TAPL is a lysosomal ATP-binding cassette transporter that translocates a broad spectrum of polypeptides from the cytoplasm into the lysosomal lumen. TAPL is a homodimeric half-transporter composed of a transmembrane domain (TMD) and a cytoplasmic nucleotide-binding domain (NBD) with an N-terminal TMD (TMD0). Here we report that, in addition to its well-known role as a peptide translocator, TAPL exhibits an ATP-dependent phosphatidylserine floppase activity that is the possible cause of its high basal ATPase activity and of the lack of coupling between ATP hydrolysis and peptide efflux. Here, we present the cryo-EM structures of mouse TAPL lacking the N-terminal TMD0 in (i) phospholipid-bound, (ii) both CHS- and 9-mer peptide-bound, and (iii) ADP·BeF3-bound states at 3.2–4.0 Å resolutions.

To obtain a nucleotide-bound structure, nanodisc-reconstituted ΔTMD0 was mixed with 9-mer peptide and Mg2+/ADP·BeF3 (mimicking the pre-hydrolysis state) before preparing cryo-EM grids. The final map has a resolution of 3.2 Å, allowing accurate modeling of the Mg2+/ADP·BeF3 complex and side chain conformations. The structure represents the typical outward-facing shape of ABC transporters, in which the two NBDs come close together and the TM helices have a very wide opening towards the lysosomal lumen (~36 Å in the longest diameter), while they are tightly packed on the cytosolic side. As a consequence, ΔTMD0 forms a V-shaped substrate transport pathway open not only to the lysosomal lumen but also laterally to the membrane luminal leaflet. We did not observe any density corresponding to lipids or peptides, indicating that both substrates are exported from ΔTMD0 prior to ATP hydrolysis. In the dimer interface, T286, S287, T290, D294, and Q298 on TM 7 interact electrostatically to stabilize the outward-facing conformation. Interestingly, the F449 residues remain protruding towards the transport pathway and pack closely together to create a latch-like architecture. Consequently, the central cavity is completely isolated from solvent, thus probably preventing the expelled substrate from re-entering. In the NBD region, the two ADP·BeF3 molecules are sandwiched between the two NBDs. The α- and β-phosphates of ADP and BeF3 interact with the Walker A motif and Q-loop from one NBD and the ABC signature motif of the other NBD.

>[2x]MRLWKAVVVTLAFVSTDVGVTTAIYAFSHLDRSLLEDIRHFNIFDSVLDLWAACLYRSCLLLGATIGVAKNSALGPRRLRASWLVITLVCLFVGIYAMAKLLLFSEVRRPIRDPWFWALFVWTYISLAASFLLWGLLATVRPDAEALEPGNEGFHGEGGAPAEQASGATLQKLLSYTKPDVAFLVAASFFLIVAALGETFLPYYTGRAIDSIVIQKSMDQFTTAVVVVCLLAIGSSLAAGIRGGIFTLVFARLNIRLRNCLFRSLVSQETSFFDENRTGDLISRLTSDTTMVSDLVSQNINIFLRNTVKVTGVVVFMFSLSWQLSLVTFMGFPIIMMVSNIYGKYYKRLSKEVQSALARASTTAEETISAMKTVRSFANEEEEAEVFLRKLQQVYKLNRKEAAAYMSYVWGSGLTLLVVQVSILYYGGHLVISGQMSSGNLIAFIIYEFVLGDCMESVGSVYSGLMQGVGAAEKVFEFIDRQPTMVHDGSLAPDHLEGRVDFENVTFTYRTRPHTQVLQNVSFSLSPGKVTALVGPSGSGKSSCVNILENFYPLQGGRVLLDGKPIGAYDHKYLHRVISLVSQEPVLFARSITDNISYGLPTVPFEMVVEAAQKANAHGFIMELQDGYSTETGEKGAQLSGGQKQRVAMARALVRNPPVLILDEATSALDAESEYLIQQAIHGNLQRHTVLIIAHRLSTVERAHLIVVLDKGRVVQQGTHQQLLAQGGLYAKLVQRQMLGLEHPLDYTASHKEPPSNTEHKA> QALLFPLCLVLYTFSTYIGNMMIQPGMLAVVEQYQAGIDWVPTSMTAYLAGGMFLQWLLGPLSDRIGRRPVMLAGVVWFIVTCLAILLAQNIEQFTLLRFLQGISLCFIGAVGYAAIQESFEEAVCIKITALMANVELIAPLLGPLVGAAWIHVLPWEGMFVLFAALAAISFFGLQRAMPETATRIGEKLSLKELGRD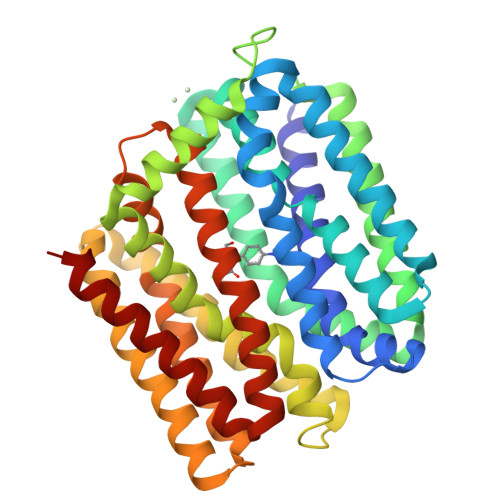YKLVLKNGRFVAGALALGFVSLPLLAWIAQSPIIIITGEQLSSYEYGLLQVPIFGALIAGNLLLARLTSRRTVRSLIIMGGWPIMIGLLVAAAATVISSHAYLWMTAGLSIYAFGIGLANAGLVRLTLFASDMSKGTVSAAMGMLQMLIFTVGIEISKHAWLNGGNGLFNLFNLVNGILWLSLMVIFLK> FSD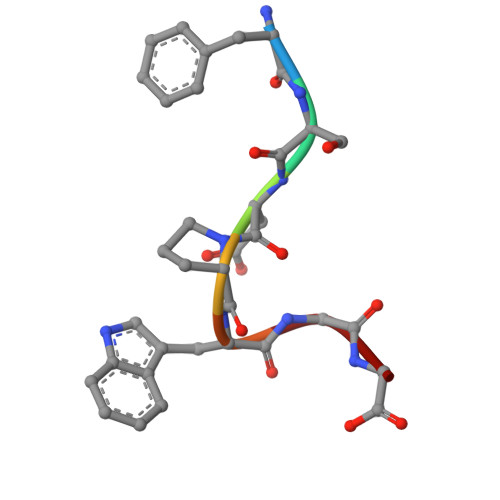PWGG> MTENILRKSDEEIQKEITARVKALESMLIEQGILTTSMIDRMAEIYENEVGPHLGAKVVVKAWTDPEFKKRLLADGTEACKELGIGGLQGEDMMWVENTDEVHHVVVCTLCSCYPWPVLGLPPNWFKEPQYRSRVVREPRQLLKEEFGFEVPPSKEIKVWDSSSEMRFVVLPQRPAGTDGWSEEELATLVTRESMIGVEPAKAVA;> MNGVYDVGGTDGLGPINRPADEPVFRAEWEKVAFAMFPATFRAGFRGLDEFRFGIEQMNPAEYLESPYYWHWIRTYIHHGVRTGKIDLEELERRTQYYRENPDAPLPEHEQKPELIEFVNQAVYGGLPASREVDRPPKFKEGDVVRFSTASPKGHARRARYVRGKTGTVVKHHGAYIYPDTAGNGLGECPEHLYTVRFTAQELWGPEGDPNSSVYYDCWEPYIELV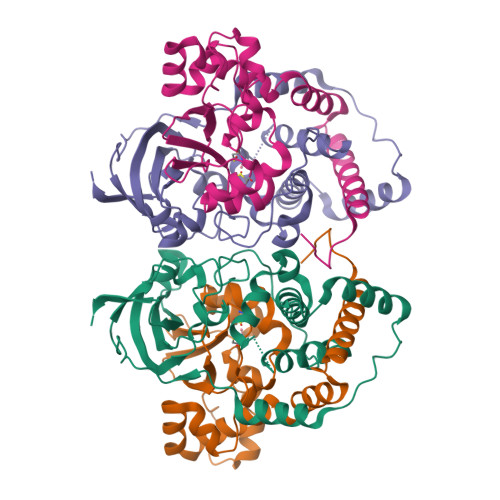DTKAAAA>[2x]AETSSATT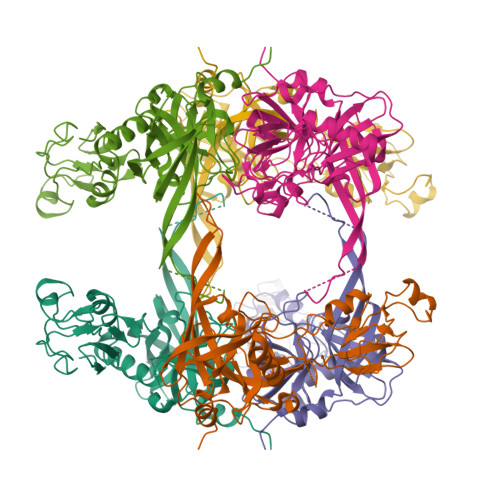AQQMPSLAPMLEKVMPSVVSINVEGSTTVNTPRMPRNFQQFFGDDSPFCQEGSPFQSSPFCQGGQGGNGGGQQQKFMALGSGVIIDADKGYVVTNNHVVDNATVIKVQLSDGRKFDAKMVGKDPRSDIALIQIQNPKNLTAIKMADSDALRVGDYTVAIGNPFGLGETVTSGIVSALGRSGLNAENYENFIQTDAAINRGNAGGALVNLNGELIGINTAILAPDGGNIGIGFAIPSNMVKNLTSQMVEYGQVKRGELGIMGTELNSELAKAMKVDAQRGAFVSQVLPNSSAAKAGIKAGDVITSLNGKPISSFAALRAQVGTMPVGSKLTLGLLRDGKQVNVNLELQQSSQNQVDSSSIFNGIEGAEMSNKGKDQGVVVNNVKTGTPAAQIGLKKGDVIIGANQQAVKNIAELRKVLDSKPSVLALNIQRGDSTIYLLMQRSHHHHHH>[2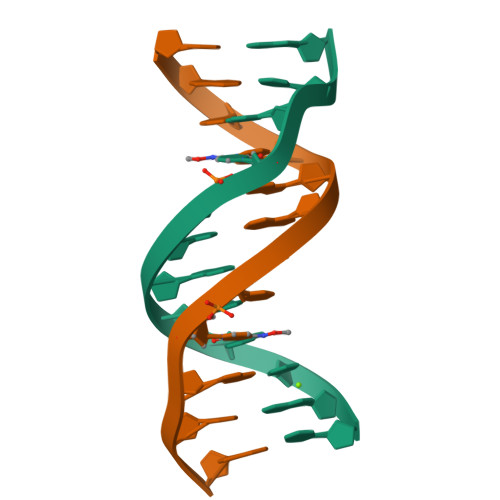x]CGCAAATTCGCG> MNTWGLIKTIFFAGSTLVFFFLLWFYNPFKHVEHYEVDEEVKAIIDNPWKKTESGKTIAEEGRELFIASCSSCHSLRYDGIYIMSVAANPKWKNIEKTSGRPVYRFGTLYKDRFFVPKDVYEAFAHDDIQGLKASLGQVPPDLSSMYLARGEGYLYQFILNPQKVLPGTTMPQLFNP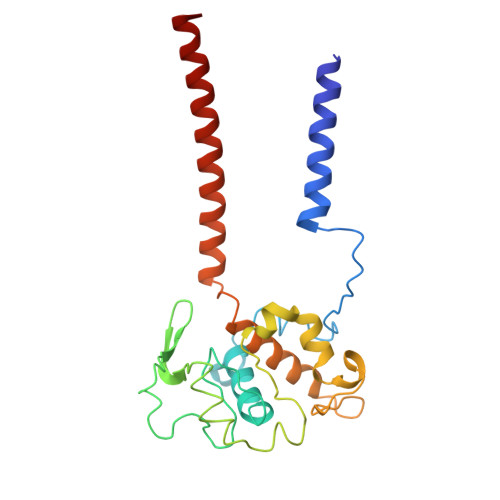QFDPQAKEKVAKIVAYMKSVNTPPPKESAKRTVMGVIVIAYFIVMGLLLWKYRENLLKRLGYH>MSAEVIDRFFKSSGAGDIETAVECFADDGQWITPDGDGLGTVHTKDQIGDLITSMNAMREKMIASGVDGKFESPIMFGENMGLVRWTVETDDGKVVNRGVDLFILSDGKIVLKDVYR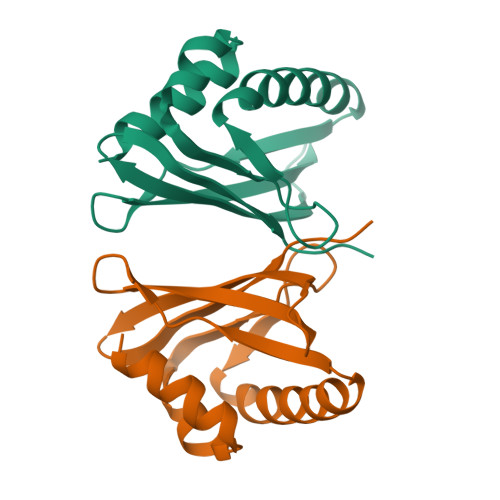KVKLAAALEHHHHHH[2x]> AAGAYDP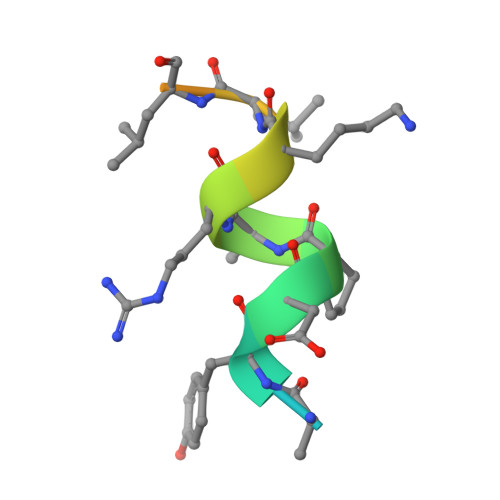ARKLLEQYAKK>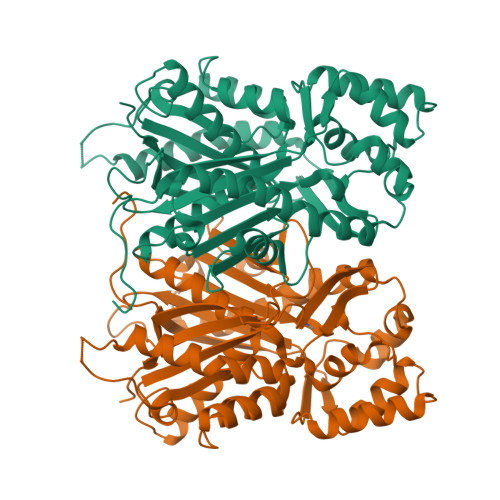 MASATIPAPAPRKMERAEGPASVLAIGTAVPPNVVYQKDYPDFYFGVTNSNHKTELKDKFQRMCDKSCVSKRHLYLTEEILKANPSLCAYWEPSLDLRQDIVVVEVPKLGKQAASAAIKEWGQPKSKITHLIFCTTSGVDMPGADWALAKLLGLRSSVKRLVLYMQGCYGGGTVLRIAKDLAENNKGARVLVVCSEITAITFRGPSDTHLDSLVGQALFGDGASALIVGSDPVPAVERAWFELHWTGSDILPNSDGAIDGHLKEVGLTFHLMKDVPAIISKNIGGILKDALAKVFPAAHDQLDSSGTTAAAPPPPTYNDLFWITHPGGPAILDQVEDRLGLRKDKLASTRAVLDQFGNMSSATVLFIMDEMRKRSVEQQLGTTGEGHEWGLLLGFGPGLTCETVVLRSVPLV>MVRRTKEEAQETRAQIIEAAERAFYKRGVARTTLADIAELAGVTRGAIYWHFNNKAELVQALLDSLHETHDHLARASESEDEVDPLGCMRKLLLQVFNELVLDARTRRINEILHHKCEFTDDMCEIRQQRQSAVLDCHKGITLALANAVRRGQLPGELDAERAAVAMFAYVDGLIRRWLLLPDSVDLLGDVEKWVDTGLDMLRLS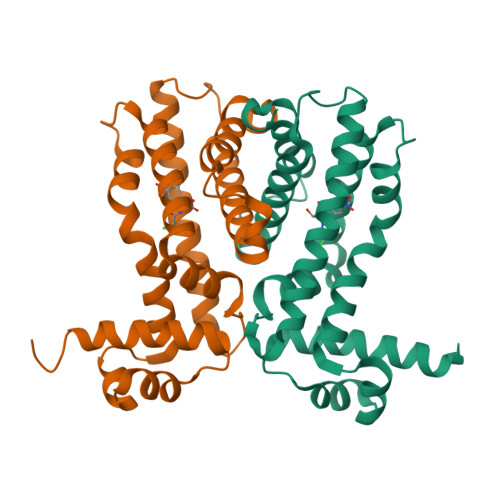PALRK[2x]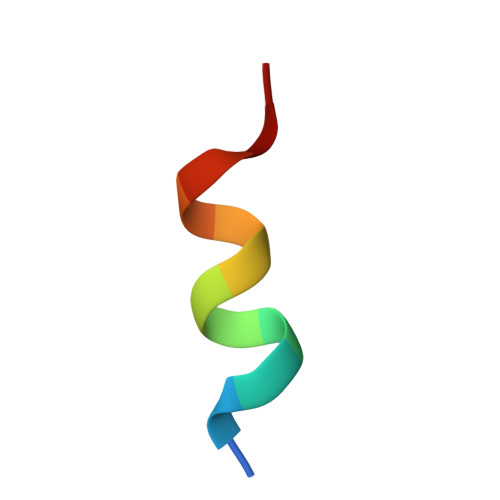> NFTLKFWDIFRK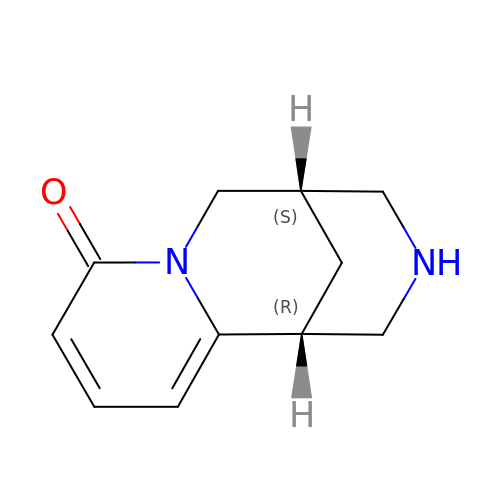(1R,5S)-1,2,3,4,5,6-HEXAHYDRO-8H-1,5-METHANOPYRIDO[1,2-A][1,5]DIAZOCIN-8-ONE | C11 H14 N2 O | ANJTVLIZGCUXLD-DTWKUNHWSA-N>ADTIVAVELDSYPNTDIGDPSYPHIGIDIKSIRSKSTARWNMQTGKVGTAHISYNSVAKRLTAVVSYSGSSSTTVSYDVDLTNVLPEWVRVGLSATTGLYKETNTILSWSFTSKLKTNSIADANALHFSFNQFTQNPKDLILQGDATTDSDGNLELTKVSSSGSPQGSSVGRALFYAPVHIWESSAVVASFDATFTFLIKSPD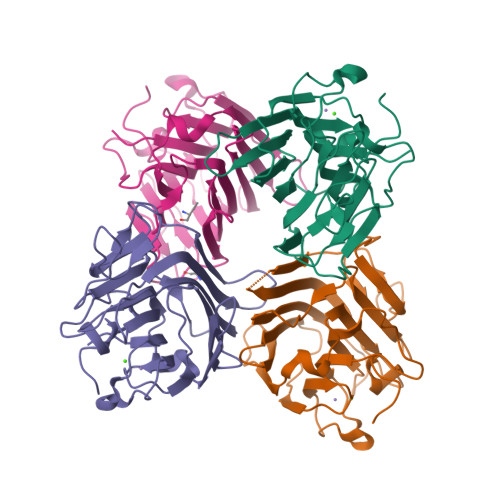SEPADGITFFIANTDTSIPSGSSGRLLGLFPDAN[4x]> DNILYSGETLSPGEFLNNGRYVFIMQEDCNLVLYDVDKPIWATNTGGLDRRCHLSMQSDGNLVVYS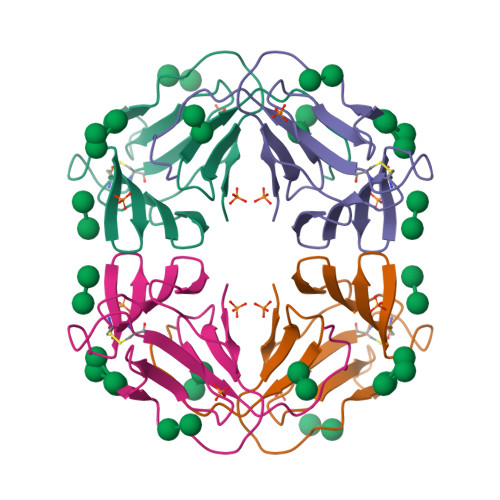PRNNPIWASNTGGENGNYVCVLQKDRNVVIYGTARWATGTNIH> MGNNASSLSELNLFSKGGVFTREQL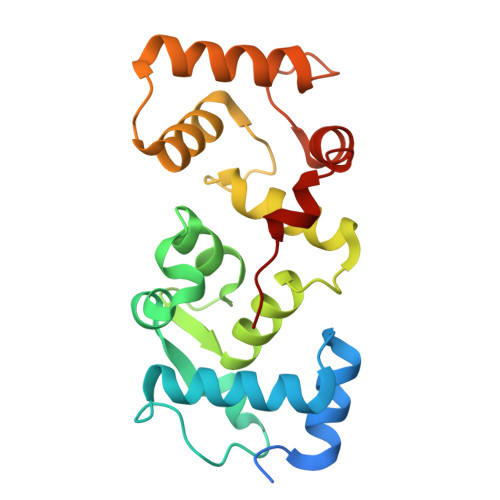DEYQDCTFFTRKDIIRLYKRFYALNPHKVPTNMQGNRPAITTLTFEEVEKMPELKENPFKRRICEVFSEDGRGNLSFDDFLDMFSVFSEMAPLQLKLKYAFRIYDYDGDELLGHDDLSKMIRSLTRDELSDVEVEFIIERIIEEADLDGDSSINFAEFEHVVSRSPDFIRTFHIRI> MDSTSTIANKIEEYLGAKSDDSKIDELLKADPSEVEYYRSGGDGDYLKNNICKITVNHSDSGKYDPCEKKLPPYDDNDQWKCQQNSSDGSGKPENICVPPRRERLCTYNLENLKFDKIRDNNAFLADVLLTARNEGEKIVQNHPDTNSSNVCNALERSFADLADIIRGTDQWKGTNSNLEKNLKQMFAKIRENDKVLQDKYPKDQKYTKLREAWWNANRQKVWEVITCGARSNDLLIKRGWRTSGKSDRKKNFELCRKCGHYEKEVPTKLDYVPQFLRWLTEWIEDFYREKQNLIDDMERHREECTREDHKSKEGTSYCSTCKDKCKKYCECVKKWKTEWENQENKYKDLYEQNKNKTSQKNTSRYDDYVKDFFEKLEANYSSLENYIKGDPYFAEYATKLSFILNPSDANNPSGETANHNDEACNCNESGISSVGQAQTSGPSSNKTCITHSSIKTNKKKECKDVKLGVRENDKDLKICVIEDTSLSGVDNCCCQDLLGILQENCSDNKRGSSSNDSCDNKNQDECQKKLEKVFASLTNGYKCDKCKSGTSRSKKKWIWKKSSGNEEGLQEEYANTIGLPPRTQSLYLGNLPKLENVCEDVKDINFDTKEKFLAGCLIVSFHEGKNLKKRYPQNKNSGNKENLCKALEYSFADYGDLIKGTSIWDNEYTKDLELNLQNNFGKLFGKYIKKNNTAEQDTSYSSLDELRESWWNTNKKYIWTAMKHGAEMNITTCNADGSVTGSGSSCDDIPTIDLIPQYLRFLQEWVENFCEQRQAKVKDVITNCKSCKESGNKCKTECKTKCKDECEKYKKFIEACGTAGGGIGTAGSPWSKRWDQIYKRYSKHIEDAKRNRKAGTKNCGTSSTTNAAASTDENKCVQSDIDSFFKHLIDIGLTTPSSYLSNVLDDNICGADKAPWTTYTTYTTTEKCNKERDKSKSQSSDTLVVVNVPSPLGNTPYRYKYACQCKIPTNEETCDDRKEYMNQWSCGSARTMKRGYKNDNYELCKYNGVDVKPTTVRSNSSKLDGNDVTFFNLFEQWNKEIQYQIEQYMTNANISCIDEKEVLDSVSDEGTPKVRGGYEDGRNNNTDQGTNCKEKCKCYKLWIEKINDQWGKQKDNYNKFRSKQIYDANKGSQNKKVVSLSNFLFFSCWEEYIQKYFNGDWSKIKNIGSDTFEFLIKKCGNNSAHGEEIFSEKLKNAEKKCKENESTDTNINKSETSCDLNATNYIRGCQSKTYDGKIFPGKGGEKQWICKDTIIHGDTNGACIPPRTQNLCVGELWDKSYGGRSNIKNDTKELLKEKIKNAIHKETELLYEYHDTGTAIISKNDKKGQKGKNDPNGLPKGFCHAVQRSFIDYKNMILGTSVNIYEHIGKLQEDIKKIIEKGTPQQKDKIGGVGSSTENVNAWWKGIEREMWDAVRCAITKINKKNNNSIFNGDECGVSPPTGNDEDQSVSWFKEWGEQFCIERLRYEQNIREACTINGKNEKKCINSKSGQGDKIQGACKRKCEKYKKYISEKKQEWDKQKTKYENKYVGKSASDLLKENYPECISANFDFIFNDNIEYKTYYPYGDYSSICSCEQVKYYKYNNAEKKNNKSLCYEKDNDMTWSKKYIKKLENGRSLEGVYVPPRRQQLCLYELFPIIIKNEEGMEKAKEELLETLQIVAEREAYYLWKQYNPTGKGIDDANKKACCAIRGSFYDLEDIIKGNDLVHDEYTKYIDSKLNEIFGSSNTNDIDTKRARTDWWENETITNGTDRKTIRQLVWDAMQSGVRYAVEEKNENFPLCMGVEHIGIAKPQFIRWLEEWTNEFCEKYTKYFEDMKSKCDPPKRADTCGDNSNIECKKACANYTNWLNPKRIEWNGMSNYYNKIYRKSNKESEDGKDYSMIMAPTVIDYLNKRCHGEINGNYICCSCKNIGAYNTTSGTVNKKLQKKETE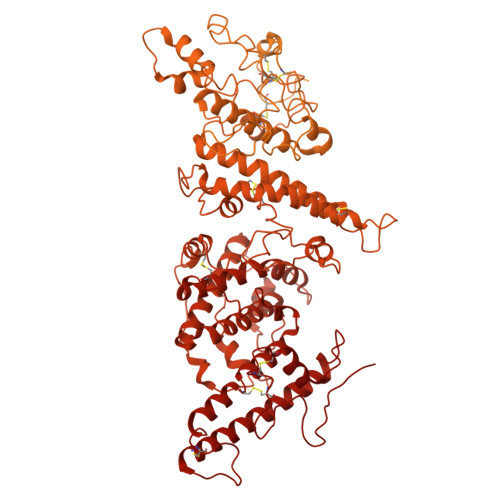CEEEKGPLDLMNEVLNKMDKKYSAHKMKCTEVYLEHVEEQLNEIDNAIKDYKLYPLDRCFDDQTKMKVCDLIADAIGCKDKTKLDELDEWNDMDLRGTYNKHKGVLIPPRRRQLCFSRIVRGPANLRSLNEFKEEILKGAQSEGKFLGNYYKEHKDKEKALEAMKNSFYDYEDIIKGTDMLTNIEFKDIKIKLDRLLEKETNNTKKAEDWWKTNKKSIWNAMLCGYKKSGNKIIDPSWCTIPTTETPPQFLRWIKEWGTNVCIQKQEHKEYVKSKCSNVTNLGAQASESNNCTSEIKKYQEWSRKRSIQWETISKRYKKYKRMDILKDVKEPDANTYLREHCSKCPCGFNDMEEMNNNEDNEKEAFKQIKEQVKIPAELEDVIYRIKHHEYDKGNDYICNKYKNIHDRMKKNNGNFVTDNFVKKSWEISNGVLIPPRRKNLFLYIDPSKICEYKKDPKLFKDFIYWSAFTEVERLKKAYGGARAKVVHAMKYSFTDIGSIIKGDDMMEKNSSDKIGKILGDTDGQNEKRKKWWDMNKYHIWESMLCGYREAEGDTETNENCRFPDIESVPQFLRWFQEWSENFCDRRQKLYDKLNSECISAECTNGSVDNSKCTHACVNYKNYILTKKTEYEIQTNKYDNEFKNKNSNDKDAPDYLKEKCNDNKCECLNKHIDDKNKTWKNPYETLEDTFKSKCDCPKPLPSPIKPDDLPPQADEPF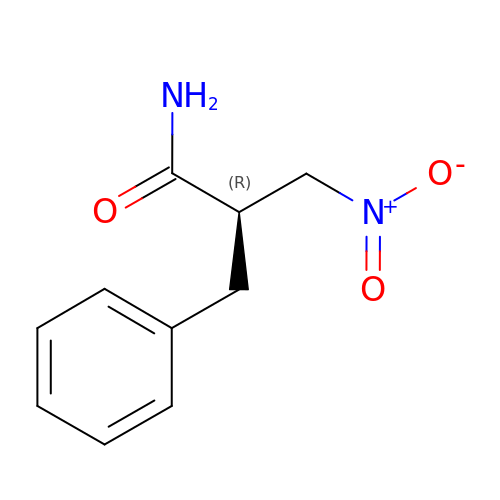(2R)-2-benzyl-3-nitropropanamide | C10 H12 N2 O3 | JJVMCABGSUOHSC-SECBINFHSA-N1,2-dihydroxy-3-(piperazine-1-sulfonyl)anthracene-9,10-dione 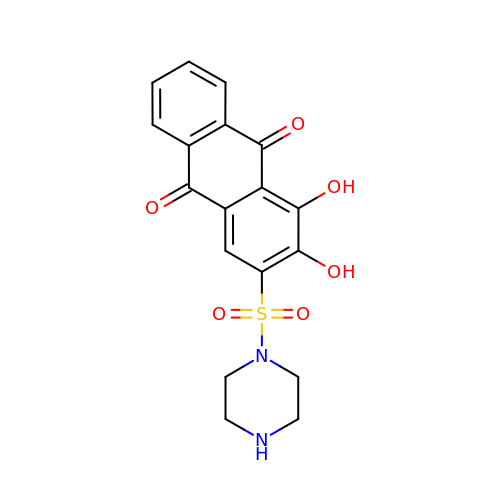| C18 H16 N2 O6 S | LUICJQQAUHLELI-UHFFFAOYSA-N> MGSVNSSPNEEFETVPDSQISGFDSPLIPTSVGSYFRDDDDDEKVHPNFISDPENDSLNSDEEFSSLENSDLNLSGAKAESGDDFDPILKRTIISKRKAPSNNEDEEIVKTPRKLVNYVPLKIFNLGDSFDDTITTTVAKLQDLKKEILDSPRSNKSIVITSNTVAKSELQKSIKFSGSIPEIYLDVVTKETISDKYKDWHFISKNCHYEQLMDLEMKDTAYSFLFGSSRSQGKVPEFVHLKCPSITNLLVLFGVNQEKCNSLKI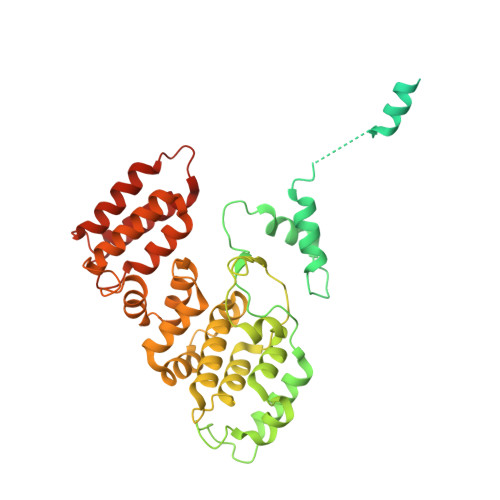NYEKKENSRYDNLCTIFPVNKMLKFLMYFYSDDDNDDVREFFLKAFICLILDRKVFNAMESDHRLCFKVLELFNEAHFINSYFEIVDKNDFFLHYRLLQIFPHLQSALLRRRFSEKQGRTETIQQNIIKEFNEFFDCKNYKNLLYFILTMYGSKFIPFGPKCQVTEYFKDCILDISNETTNDVEISILKGILNLFSKIR>[3x]HHHHHHFNLPPGNYKKPKLLYCSNGGHFLRILPDGTVDGTRDRSDQHIQLQLSAESVGEVYIKSTETGQYLAMDTDGL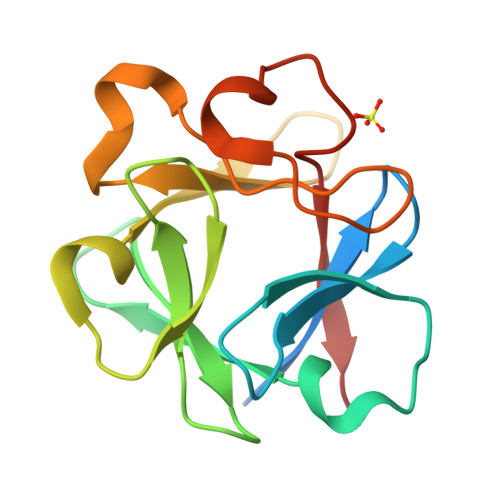LYGSQTPNEECLFLERLEENGYNTYISKKHAEKNWFVGLKKNGSCKRGPRTHYGQKAILFLPLPVSSD>[2x]ADQSFLWNVFQRVDKDRSGVISDTELQQALSNGTWTPFNPVTVRSIISMFDRENKAGVNFSEFTGVWKYITDWQNVFRTYDRDNSGMID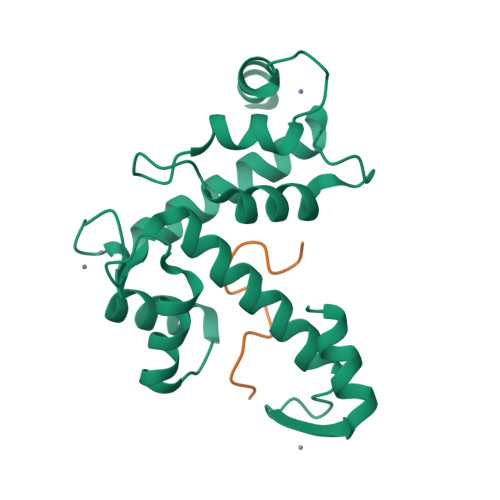KNELKQALSGFGYRLSDQFHDILIRKFDRQGRGQIAFDDFIQGCIVLQRLTDIFRRYDTDQDGWIQVSYEQYLSMVFSIV;>[2x]QGPPYPTYPGYPGYSQ The third step in the sialic acid catabolic pathway is mediated by the enzyme N-acetylmannosamine-6-phosphate 2-epimerase (NanE), which catalyzes an inversion of stereochemistry at the C2 position of N-acetylmannosamine-6-phosphate (ManNAc-6P), yielding N-acetylglucosamine-6-phosphate (GlcNAc-6P). The crystal structure of NanE from Staphylococcus aureus, which comprises a triosephosphate isomerase barrel fold with an unusual dimeric architecture, was solved with both natural and modified substrates. NanE is essential for the growth of S. aureus in media containing N-acetylneuraminic acid as the sole carbon source and has a highly conserved active site across both Gram-positive and Gram-negative bacteria. Based on our structural and kinetic data, we propose that NanE performs its epimerization reaction using a novel proton displacement mechanism mediated by the substrate.

As Glu180 forms a short hydrogen bond with the C5 hydroxyl of the substrate, we generated SaNanE-Glu180Ala and tested the effect of this substitution on activity. We found that SaNanE-Glu180Ala retained ∼0.05% activity, but the KM was similar to that of the wildtype enzyme, suggesting that Glu180 plays a role in the catalytic mechanism. The single-residue substitution made no change to the overall structure or the conserved active-site residues. The salt bridge between Arg40 and Asp124 was preserved to stabilize the enolate, and the KM was similar to wildtype SaNanE, indicating that the short bond to the C5 hydroxyl makes only a minor contribution to substrate binding. This suggests that the reduction in kcat is due to the loss of Glu180 in the reaction mechanism rather than a compromise in substrate binding. The residual activity of the enzyme may result from an active-site water molecule that acts in place of Glu180 during catalysis, a phenomenon we have seen before in another unrelated TIM-barrel enzyme, dihydrodipicolinate synthase.

>[2x]MLPHGLIVSCQALPDEPLHSSFIMSKMALAAYEGGAVGIRANTKEDILAIKETVDLPVIGIVKRDYDHSDVFITATSKEVDELIESQCEVIALDATLQQRPKETLDELVSYIRTHAPNVEIMADIATVEEAKNAARLGFDYIGTTLHGYTSYTQGQLLYQNDFQFLKDVLQSVDAKVIAAGNVITPDMYKRVMDLGVHCSVVGGAITRPKEITKRFVQIMED> QSVCAGTENKLSSLSDLEQQYRALRKYYENCEVVMGNLEITSIEHNRDLSFLRSVREVTGYVLVALNQFRYLPLENLRIIRGTKLYEDRYALAIFLNYRKDGNFGLQELGLKNLTEILNGGVYVDQNKFLCYADTIHWQDIVRNPWPSNLTLVSTNGSSGCGRCHKSCTGRCWGPTENHCQTLTRTVCAEQCDGRCYGPYVSDCCHRECAGGCSGPKDTDCFACMNFNDSGACVTQCPQTFVYNPTTFQLEHNFNAKYTYGAFCVKKCPHNFVVDSSSCVRACPSSKMEVEENGIKMCKPCTDICPKACDGIGTGSLMSAQTVDSSNIDKFINCTKINGNLIFLVTGIHGDPYNAIEAIDPEKLNVFRTVREITGFLNIQSWPPNMTDFSVFSNLVT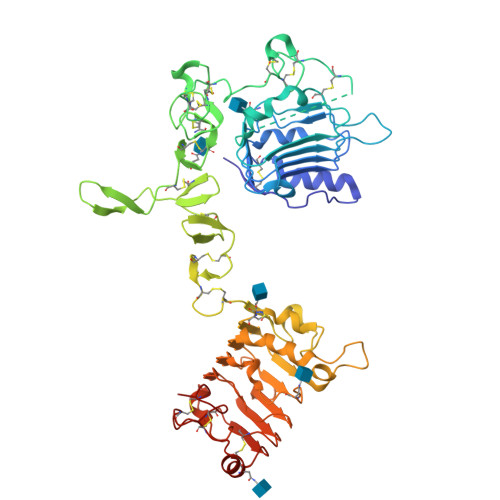IGGRVLYSGLSLLILKQQGITSLQFQSLKEISAGNIYITDNSNLCYYHTINWTTLFSTINQRIVIRDNRKAENCTAEGMVCNHLCSSDGCWGPGPDQCLS1-{4-[3-(4-fluorophenyl)-1-methyl-1H-pyrazol-4-yl]pyridin-2-yl}-N-methylmethanamine | C17 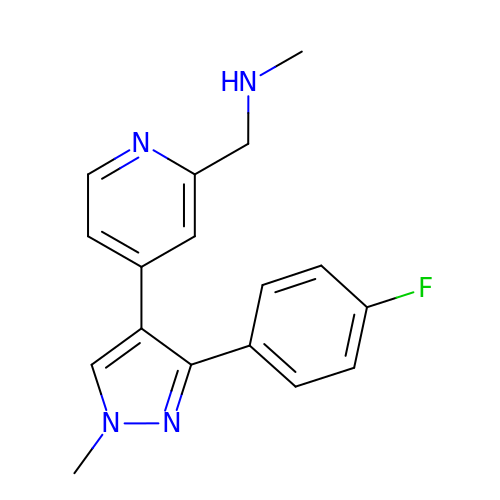H17 F N4 | UEPOHWWKVBWCFV-UHFFFAOYSA-N>[2x]MAQQKKTIAVVNATGRQAASLIRVAAAVGHHVRAQVHSLKGLIAEELQAIPNVTLFQGPLLNNVPLMDTLFEGAHLAFINTTSQAGDEIAIGKDLADAAKRAGTIQHYIYSSMPDHSLYGPWPAVPMWAPKFTVENYVRQLGLPSTFVYAGIYNNNFTSLPYPLFQMELMPDGTFEWHAPFDPDIPLPWLDAEHDVGPALLQIFKDGPQKWNGHRIALTFETLS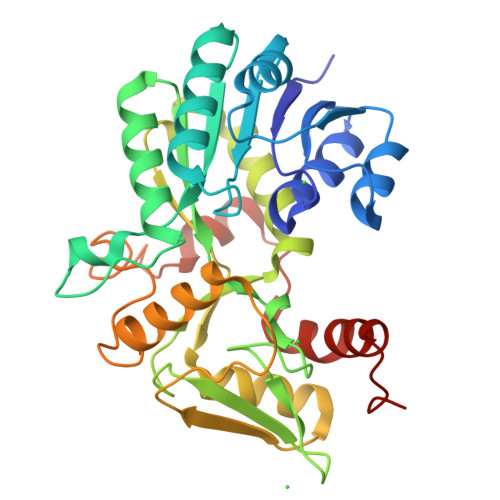PVQVCAAFSRALNRRVTYVQVPKVEIKVNIPVGYREQLEAIEVVFGEHKAPYFPLPEFSRPAAGSPKGLGPANGKGAGAGMMQGPGGVISQRVTDEARKLWSGWRDMEEYAREVFPIEEEANGLDWML The binding of the plant phytohormone Abscisic acid (ABA) to the family of ABA receptors (PYR/PYL/RCAR) triggers plant responses to abiotic stress. In the resting state, the PYR/PYL receptors are monomers or dimers and display a wide empty ABA binding cavity flanked by two highly conserved loops, named as gate loop and latch loop. To investigate this issue, we have selected as a model SlPYL1 which is a tomato dimeric receptor with known structure that is involved in the induction of stress responsive genes and drought tolerance. Interestingly, the analysis of the structure of SlPYL1 shows that Glu 151 is not involved in the dimerization interface or interacting with ABA; rather, it is located in the latch loop.

To investigate the relevance of this amino acid on the receptor function, we generated a mutated version of SlPYL1 harboring a Glu 151 to Asp substitution (SlPYL1 E151D) at the latch and studied its biochemical properties and compared them with those of the native protein. The overall structures of the apo and ABA bound forms of SlPYL1 E151D are nearly identical to that of WT protein with the differences confined to the area of the mutated residue. The Root Mean Squared Deviation for 191 Calpha atoms are of 0.33A and 0.20A for the apo and ABA bound forms, respectively. In addition, the ABA bound structure shows that Asp 151 carboxylate is hydrogen bonded to the NH of Thr 128 at the C-terminal end of the gate loop. This hydrogen bond is not present in the native structure and might account for the increased stability of the mutant protein in complex with ABA with respect to that observed for the native protein. In addition, the analysis of the ABA bound structures of SlPYL1 E151D and SlPYL1 showed that Glu 151 replacement to Asp leads to the formation of an additional hydrogen bond linking Asp 151 at the latch and Thr 110 at the gate. This would explain our data showing that the ABA bound form of SlPYL1 E151D displays increased stability as compared with that of SlPYL1. Interestingly, there is a reduction of the RMSD as a result of ABA binding, that indicates that hormone binding stabilizes the entire gate loop despite it does not make any direct contact with ABA. However, the degree of such stabilization is higher in the mutant protein. The complex nature of the denaturation profiles obtained without or at low concentrations of ABA hinders the calculation of Ti, however, SlPYL1 E151D protein displays larger Ti than the WT in the presence of 4 mM ABA, showing that the Asp side chain is involved in the stabilization of the protein.

> MDNKPETSLDNPVHQRSEPGSETGSSLSTITTHHLTVPPGLTPEEFQELSSSIAEFHSYRINPGQCSSLLAQRIHAPVETVWTVVRRFDKPQTYKHFIKSCSVGEDFRMTVGSTRDVTVISGLPAATSTERLDILDDDRHVTGFSIIGGDHRLRNYRSVTTVHGFERDGEIWTVVLESYVVDVPEGNTEEDTRLFADTVVKLNLQKLASVTETLAREAGNGSVNSRDASHRS>GAMGSWNPKYDTRTLWTTPDTSPNCTIAQDKDSKLTLVLTKCGSQILANVSLIVVAGKYHIINNKTNPKIKSFTIKLLFNKNGVLLDNSNLGKAYWNFRSGNSNVSTAYEKAIGFMPNLVAYPKPSNSKKYARDIVYGTIYLGGKPDQPAVIKTTFNQETGCEYSITFNFSWSKTYENVEFET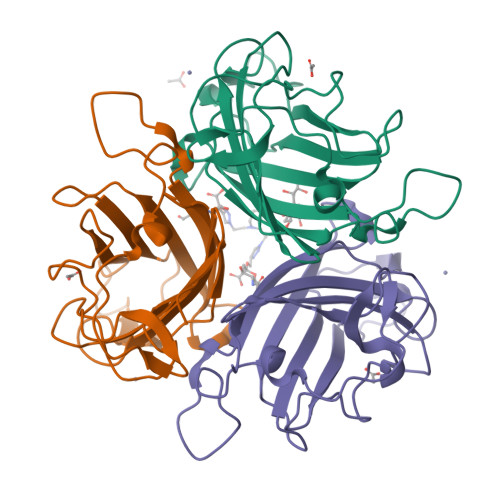TSFTFSYIAQE[3x]BgaA is specific for galactose β-1,4-linked to glucose or GlcNAc [lactose or N-acetyllactosamine (LacNAc) motifs, respectively] found in glycoconjugates. The N-terminal region of BgaA comprising amino acid residues 138–993 has amino acid sequence identity with GH family 2 enzymes. Through detailed structural and functional analyses the molecular basis for the catalytic specificity of BgaA is defined and this activity is demonstrated as critical for the ability of pneumococci to utilize complex N-linked glycans as a carbon source and protect the bacterium from opsonophagocytic killing. Further analyses also revealed the presence of non-catalytic CBMs within the C-terminal region of BgaA that mediate adherence to host cell surface LacNAc and/or lactose.

The X-ray crystal structures of a catalytically active fragment of BgaA was determined to 2.7 Å resolution (data not shown) and an inactive Glu645Gln nucleophile mutant in complex with unhydrolyzed LacNAc to 2.2 Å resolution. This polypeptide had five distinct domains, four with immunoglobulin (Ig)-like folds that are arranged to create a nest in which the central (α/β)8-barrel domain III sits. The catalytic site of BgaA resides in a pocket located at the center of domain III and makes a series of direct and water-mediated hydrogen bonds with both residues of the disaccharide while the a-face of the GlcNAc residues lies parallel to Trp685 in a classical carbohydrate ring-aromatic amino acid sidechain interaction. The LacNAc in this complex does not fully engage the catalytic residues: neither Glu564, the acid base, nor Gln645, mutated from the glutamic acid that would normally act as the nucleophile, are appropriately positioned to perform a catalytic function. This “shallow” mode of substrate binding representing an active site loading step is the same as that observed for Escherichia coli LacZ Glu537Gln mutant in complex with lactose. The catalytically non-productive loading mode appears to provide BgaA with its substrate specificity through a pre-(−1)-subsite that recognizes terminal galactose residues and a preceding pre-(+1)-subsite that accommodates the β-1,4-linked GlcNAc residue through primary interactions with Trp685 and a series of hydrogen bonds between O6 of this sugar residue and a tailored pocket. The steric constraints imposed by this architecture legislate against β-1,6-linked GlcNAc, with its longer overall length, and β-1,3-linked GlcNAc, where the 2-acetamido group would clash with the O6-specific pocket in the active site. Indeed, BgaA has insignificant activity on these sugars. This substrate-loading mode does not, however, suggest a mechanism for discrimination between lactose and LacNAc, where the latter is preferred by a factor of ∼10-fold.

> AVTNEEVNQMIEDRKVDFNQNWYFKLNANSKEAIKPDADVSTWKKLDLPYDWSIFNDFDHESPAQNEGGQLNGGEAWYRKTFKLDEKDLKKNVRLTFDGVYMDSQVYVNGQLVGHYPNGYNQFSYDITKYLQKDGRENVIAVHAVNKQPSSRWYSGSGIYRDVTLQVTDKVHVEKNGTTILTPKLEEQQHGKVETHVTSKIVNTDDKDHELVAEYQIVERGGHAVTGLVRTASRTLKAHESTSLDAILEVERPKLWTVLNDKPALYELITRVYRDGQLVDAKKDLFGYRYYHWTPNEGFSLNGERIKFHGVSLHHDHGALGAEENYKAEYRRLKQMKEMGVNSIRTTHNPASEQTLQIAAELGLLVQEEAFDTWYGGKKPYDYGRFFEKDATHPEARKGEKWSDFDLRTMVERGKNNPAIFMWSIGNEIGEANGDAHSLATVKRLVKVIKDVDKTRYVTMGADKFRFGNGSGGHEKIADELDAVGFNYSEDNYKALRAKHPKWLIYGSQTSSATRTRGSYYRPERELKHSNGPERNYEQSDYGNDRVGWGKTATASWTFDRDNAGYAGQFIWTGTDYIGEPTPWHNQNQTPVKSSYFGIVDTAGIPKHDFYLYQSQWVSVKKKPMVHLLPHWNWENKELASKVADSEGKIPVRAYSNASSVELFLNGKSLGLKTFNKKQTSDGRTYQEGANANELYLEWKVAYQPGTLEAIARDESGKEIARDKITTAGKPAAVRLIKEDHAIAADGKDLTYIYYEIVDSQGNVVPTANNLVRFQLHGQGQLVGVDNGEQASRERYKAQADGSWIRKAFNGKGVAIVKSTEQAGKFTLTAHSDLLKSNQVTVFTGKKEG>[2x]MQRNTLKHRILITGGAGFIGGHLARALVASGEEVTVLDDLRVPPMIPPEGTGKFLEKPVLELEERDLSDVRLVYHLASHKSVPRSFKQPLDYLDNVDSGRHLLALCTSVGVPKVVVGSTCEVYGQADTLPTPEDSPLSPRSPY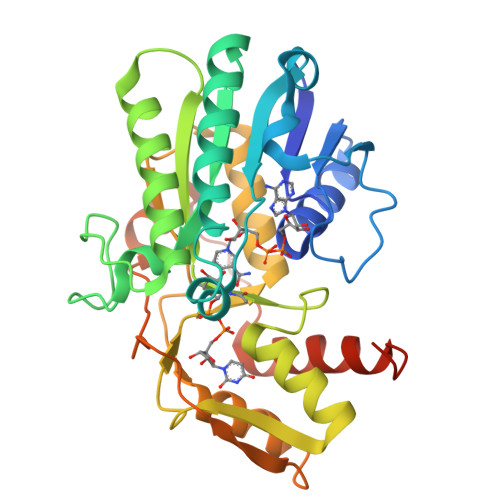AASKVGLEMVAGAHQRASVAPEVGIVRFFNVYGPGERPDALVPRLCANLLTRNELPVEGDGEQRRDFTYITDVVDKLVALANRPLPSVVNFGSGQSLSVNDVIRILQATSPAAEVARKQPRPNEITEFRADTALQTRQIGERSGGIGIEEGIRLTLEWWQSRDLDDIRQRIFQEEGAD> GIKVFLHERELWLKFHEVGTEMIITKAGRRMFPSYKVKVTGLNPKTKYILLMDIVPADDHRYKFADNKWSVTGKAEPAMPGRLYVHPDSPATGAHWMRQLVSFQKLKLTNNHLDPFGHIILNSMHKYQPRLHIVKADE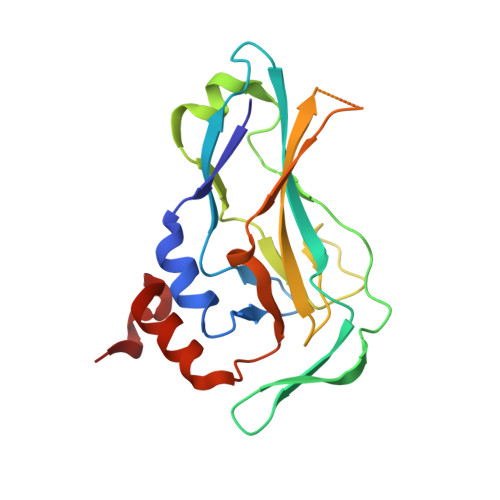NNGFGSKNTAFCTHVFPETAFIAVTSYQNHKITQLKIENNPFAKGFRG>[10x]MTAPRSWAPTTRARGDTEALCSPEDGWVKVHPTPGTMLFREILHGQLGYTEGQGVYNVVRSSEATTRQLQAAIFHALLNATTYRDLEADWLGHVAARGLQPQRLVRRYRNAREADIAGVAERVFDTWRNTLRTTLLDFAHGLVACFAPGGPSGPSSFP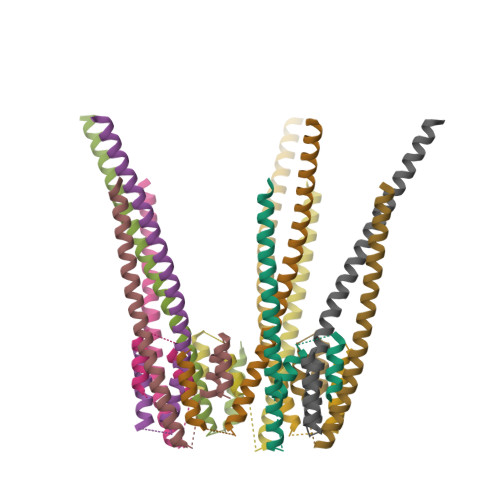KYIDWLTCLGLVPILRKRQEGGVTQGLRAFLKQHPLTRQLATVAEAAERAGPGFFELALAFDSTRVADYDRVYIYYNHRRGDWLVRDPISGQRGECLVLWPPLWTGDRLVFDSPVQRLFPEIVACHSLREHAHVCRLRNTASVKVLLGRKSDSERGVAGAARVVNKVLGEDDETKAGSAASRLVRLIINMKGMRHVGDINDTVRSYLDEAGGHLIDAPAVDGTLPGFGKGGNSRGSAGQDQGGRAPQLRQAFRTAVVNNINGVLEGYINNLFGTIERLRETNAGLATQLQERDRELRRATAGALERQQRAADLAAESVTGGCGSRPAGADLLRADYDIIDVSKSMDDDTYVANSFQHPYIPSYAQDLERLSRLWEHELVRCFKILCHRNNQGQETSISYSSGAIAAFVAPYFESVLRAPRVGAPITGSDVILGEEELWDAVFKKTRLQTYLTDIAALFVADVQHAALPPPPSPVGADFRPGASPRGRSRSRSPGRTAPGAPDQGGGIGHRDGRRDGRR>GSMEEPEESLNTLKLCSPEEFTRLCREKTQEIYPIKEANGRTRKALIICNTEFKHLSLRYGANFDIIGMKGLLEDLGYDVVVKEELTAEGMESEMKDFAALSEHQTSDSTFLVLMSHGTLHGICGTMHSEKTPDVLQYDT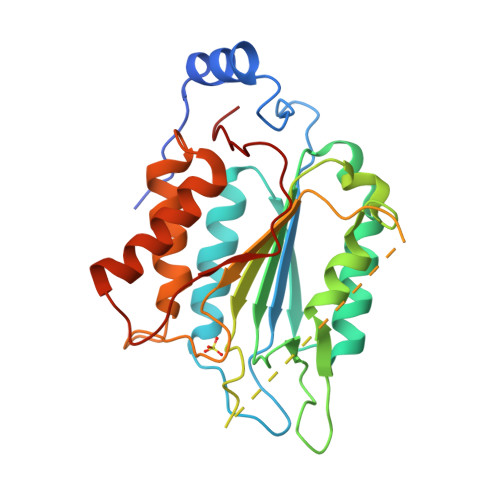IYQIFNNCHCPGLRDKPKVIIVQAARGGNSGEMWIRESSKPQLCRGVDLPRNMEADAVKLSHVEKDFIAFYSTTPHHLSYRDKTGGSYFITRLISCFRKHACSCHLFDIFLKVQQSFEKASIHSQMPTIDRATLTRYFYLFPGN[4x]>GHMFGSINLASSLSVDAPGLQNQIDELSSFSDAPSPSVTRVLYTDKDVSARRYVKNLMALAGLTVREDAVGNIFGKWDGLEPNLPAVATGSHIDAIPYSGKYDGVVGVLGAIEAINVLKRSGFKPKRSLEIILFTSAEPTRFGISCLGSRLLAGSKELAEALKTTVVDGQNVSFIEAARSAGYAEDKDDDLSSVFLKKGSYFAFLELHIEQGPILEDEGLDIGVVTAIAAPASLKVEFEGNGGHAGAVLMPYRNDAGLAAAELALAVEKHVLESESIDTVGTVGILELHPGAINSIPSKSHLEIDTRDIDEARRNTVIKKIQESANTIAKKRKVKLSEFKIVNQDPPALSDKLVIKK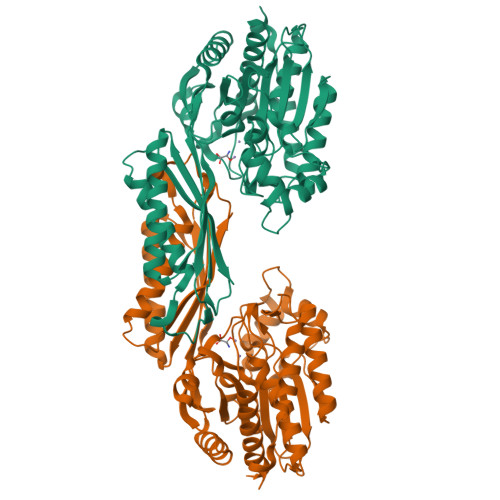MAEAATELNLSHKMMISRAYHDSLFMARISPMGMIFIPCYKGYSHKPEEYSSPEDMANGVKVLSLTLAKLSLD[2x]> 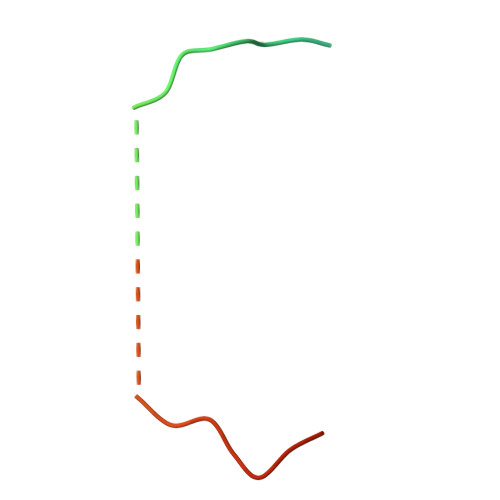GSQSQLSHQDLQLVKGAMAATYSALNSSKPTPQLKPIESSILAQRRVRKLPSTTL>MPMQMFMQVYDEIQMFLLEELELKFDMDPNRVRYLRKMMDTTCLGGKYNRGLTVIDVAESLLS[2x];>[2x]DGARRKRVLHDACVCGWMIEFLQAHYLVEDDIMDNSVTRRGKPCWYRHPDVTVQCAINDGLLLKSWTHMMAMHFFADRPFLQDLLCRFNRVDYTTAVGQLYDVTSMFDSNKLDPDVSQPTTTDFAEFTLSNYKRIVKYKTAYYTYLLPLVMGLIVSEALPTVDMGVTEELAMLMGEYFQVQD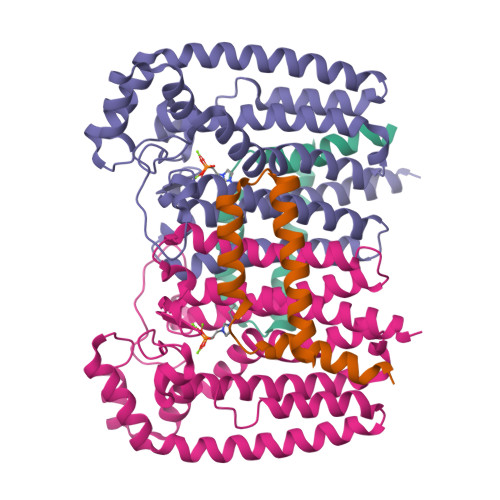DVMDCFTPPERLGKVGTDIQDAKCSWLAVTFLAKASSAQVAEFKANYGSGDSEKVATVRRLYEEADLQGDYVAYEAAVAEQVKELIEKLRLCSPGFAASVETLWGKTYKRQK> MTALTESSTSKFVKINEKGFSDFNIHYNEAGNGETVIMLHGGGPGAGGWSNYYRNVGPFVDAGYRVILKDSPGFNKSDAVVMDEQRGLVNARAVKGLMDALDIDRAHLVGNAMGGATALNFALEYPDRIGKLILMGPGGLGPSMFAPMPMEGIKLLFKLYAEPSYETLKQMLQVFLYDQSLITEELLQGRWEAIQRQPEHLKNFLISAQKAPLSTWDVTARLGEIKAKTFITWGRDDRFVPLDHGLKLLWNIDDARLHVFSKCGQWAQWEHADEFNRLVI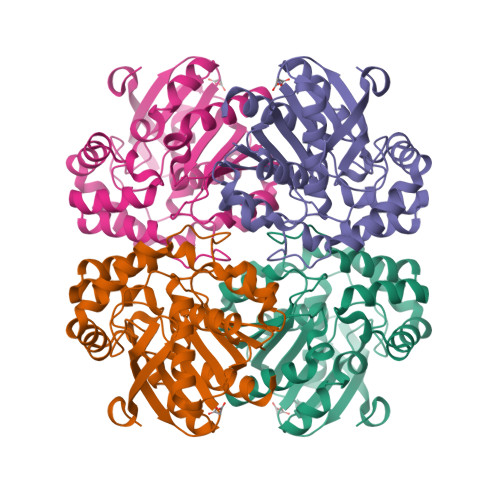DFLRHA> NNDHINLKVAGQDGSVVQFKIKRHTPLSKLMKAYCERQGLSMRQIRFRFDGQPINETDTPAQLEMEDEDTI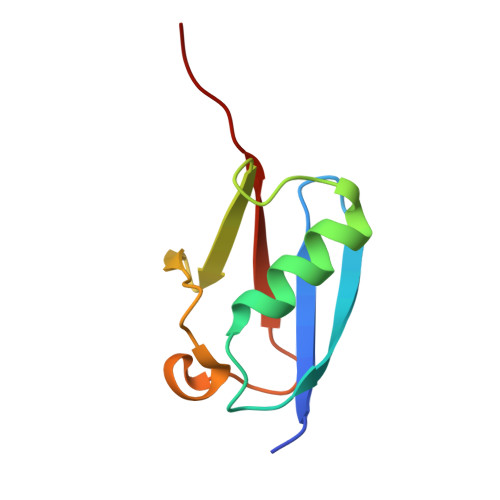DVFQQQTGG>MRGSHHHHHHGSSYQIAVLAGDGIGPEVMAEARKVLAAVEKRFDLSIEYSEYDVGGAAIDNHGCPLPEATLKGCEAADAVLFGSVGGPKWEHLPPND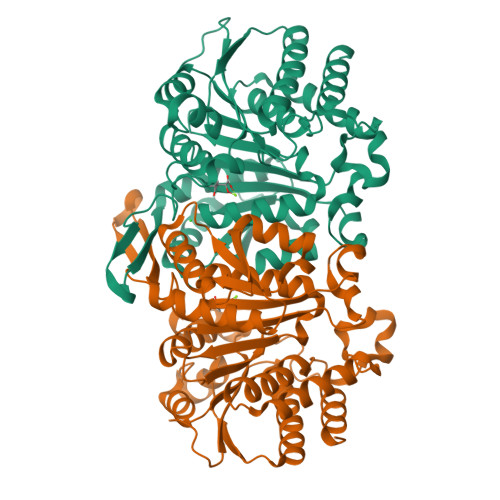QPERGALLPLRGHFELFCNMRPAKLHPGLEHMSPLRSDISEKGFDILCVRELTGGIYFGKPKGRQGEGENEEAFDTMRYSRKEIRRIAKIAFESAQGRRKKVTSVDKANVLACSVLWREVVEEVAKDYPDVELEHIYIDNATMQLLRRPNEFDVMLCSNLFGDIVSDEIAMLTGSMGLLASISMNSQGFGMYEPAGGSAPDIAGQGIANPVAQILSAALLLRHSLKLEDAALAIEAAVSKALSDGYLTCELLPASERSQAKSTSQMGDYIAQAIAEGV[2x]> MSKTDYILRALSKISHKRWEHYIINRVVHTLDDPDIEFVCQQCIRKEGHLGKIYLADLLFPQLNLYLEIDEAHHDSNDARKADAVRRLDIVEATGFQEERIPASNITLSEVNKLVDEFVRLVKDKKEELENQGLFFRWDYDERYSAKKHINTGYMAVGPNSVFRYHRDALQCFGYRREGHHQSGGWALPAEVAQSIGLTGRVMVWFPRLYEAGEWKNALSADGNKITEQSLNATRNYQETWDYRIVMAHSRDELNRTLYRFLGVFAIDVDKSSDEVKVFSRVYSRV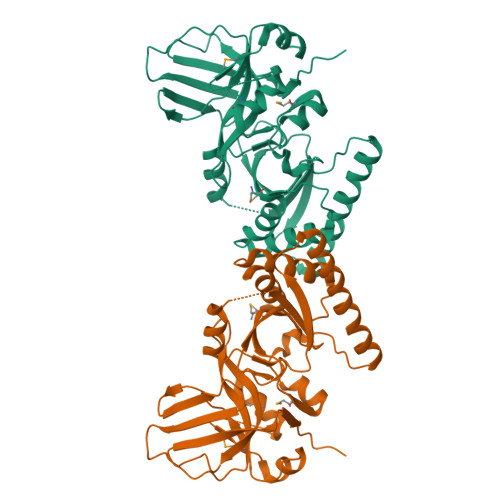NVYRSQN>ADTCYNDVALDCGITSNSLALPRCNAVYGEYGSHGNVATELQAYAKLHLERSYDYLLSAAYFNNYQTNRAGFSKLFKKLSDEAWSKTIDIIKHVTKRGDKMNFDQHSTMKTERKNYTAENHELEALAKALDTQKELAERAFYIHREATRNSQHLHDPEIAQYLEEEFIEDHAEKIRTLAGHTSDLKKFITANNGHDLSLALYVFDEYLQKTV[12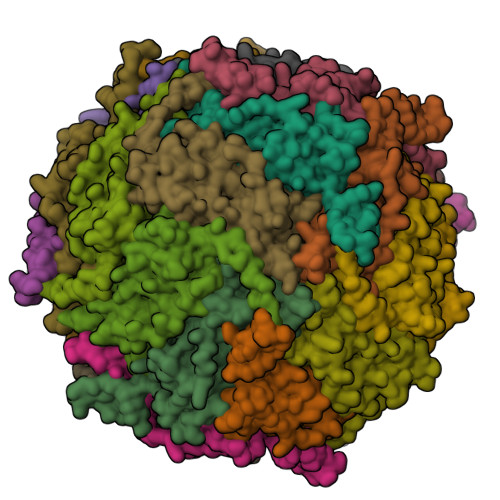x];>[12x]TQCNVNPVQIPKDWITMHRSCRNSMRQQIQMEVGASLQYLAMGAHFSKDVVNRPGFAQLFFDAASEEREHAMKLIEYLLMRGELTNDVSSLLQVRPPTRSSWKGGVEALEHALSMESDVTKSIRNVIKACEDDSEFNDYHLVDYLTGDFLEEQYKGQRDLAGKASTLKKLMDRHEALGEFIFDKKLLGIDV>SLHSPGKAFRAALTKE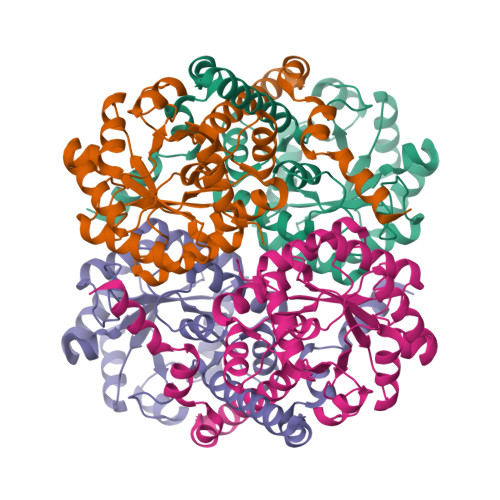NPLQIVGTINANHALLAQRAGYQAIYLSGGGVAAGSLGLPDLGISTLDDVLTDIRRITDVCSLPLLVDADIGFGSSAFNVARTVKSMIKAGAAGLHIEDQVGAKRCGHRPNKAIVSKEEMVDRIRAAVDAKTDPDFVIMARTDALAVEGLDAAIERAQAYVEAGAEMLFPEAITELAMYRQFADAVQVPILANITEFGATPLFTTDELRSAHVAMALYPLSAFRAMNRAAEHVYNVLRQEGTQKSVIDTMQTRNELYESINYYQYEEKLDNLFARSQVK[2x]Other regions in the spike S2 subunit, such as the stem helix and the segment encompassing residues 815-823 adjacent to the fusion peptide, are highly conserved across sarbecoviruses and are recognized by broadly reactive antibodies, providing hope that vaccines targeting these epitopes could offer protection against both current and emergent viruses. Here we employ computational modeling to design scaffolded immunogens that display the spike 815-823 peptide and the stem helix epitopes without the distracting and immunodominant receptor binding domain. Unlike peptide-based immunogens that can sample diverse epitope conformations, epitope scaffolds are meant to present only the antibody-bound conformation of the target epitope on their surface, which typically leads to higher antibody affinity and the elicitation of antibodies specific for the structure of the target epitope.

Given the failure of side chain grafting to produce epitope scaffolds that engage the CC40.8 mAb, we employed an alternative design technique, termed backbone grafting. Here, rather than transplanting only the epitope-specific residues onto a preexisting scaffold backbone which is otherwise unchanged, an entire region of the parent scaffold backbone is replaced with the backbone of the secondary structure containing the desired epitope. This allows the grafting of more complex epitopes that have no existing structural match, such as the CC40.8 S2-helix epitope. Next, we optimized the sequence of the S2hlx-Ex designs using ProteinMPNN21, a recently described deep learning algorithm that takes a protein structure as input and generates amino acid sequences that are predicted to generate the same fold. Analysis of a high-resolution (2.3 Å) crystal structure of unbound S2hlx-Ex19 further confirmed the successful transplantation of the CC40.8 mAb epitope. As expected, the grafted epitope region in S2hlx-Ex19 diverged considerably from the backbone region it replaced in the parent scaffold (backbone RMSD = 5.8 Å), with the epitope adopting a more exposed conformation that allows for antibody engagement. This conformational change was likely facilitated by introducing two aromatic residues (Tyr62 and Phe66) under the epitope helix, which effectively pushed the epitope segment away from the rest of the protein core. Interestingly, the epitope conformation on S2hlx-Ex19 was almost identical to that present on the prefusion stem helix, rather than the more extended one induced by CC40.8. Nevertheless, given the high affinity of S2hlx-Ex19 for CC40.8 (KD = 6.7 nM), it is likely that the antibody can readily induce the necessary conformation upon binding. Interestingly, the stem helix immunogen S2hlx-Ex19, which bound with affinities for CC40.8 and S2P6 similar to those of the native spike, displays the epitope at the N-terminus of the scaffold.

>[2x]MNLDSFKEELDDYFKEKIVKEFEKLCKELISKYEVKKPTPSPEIKKICEYLKKKHEELKDKYPEEFVKEIFKKMWEVFKKELSKQLKKLGVTNDGGEKYKIVKEDLNYLVDVIKSLEGLSDLDLNWEEIWNLEHHHHHH(2R)-2-[[3-[[3-[(Z)-(2,4-dioxo-1,3-thiazolidin-5-ylidene)methyl]phenoxy]methyl]phenyl]carbonylamino]pentanedioic acid | C23 H20 N2 O8 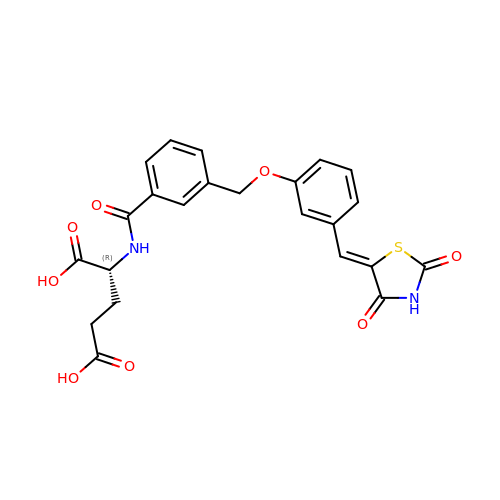S | LTRBYYDVMAAOIG-LVSMMTLPSA-N>[2x]STKKKPLTQEQLEDARRLKAIYEKKKNELGLSQESVADKMGMGQSGVGALFNGINALNAYNAALLAKILKVSVEEFSPSIAREIYEMYEAVSMQPSLRSE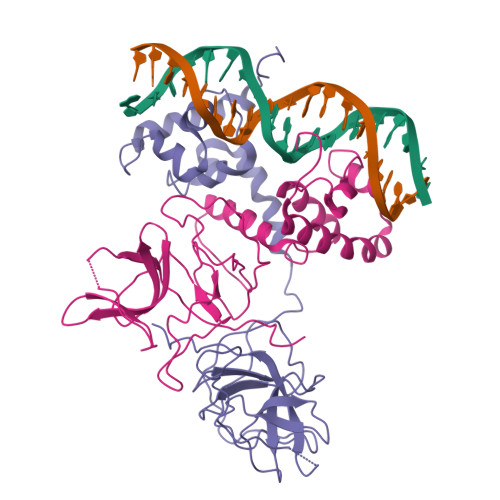YEYPVFSHVQAGMFSPELRTFTKGDAERWVSTTKKASDSAFWLEVEGNSMTAPTGSKPSFPDGMLILVDPEQAVEPGDFCIARLGGDEFTFKKLIRGSGQVFLQPLNPQYPMIPCNESCSVVGKVIASQWPEETFG CETYL-TRIMETHYL-AMMONIUM | C19 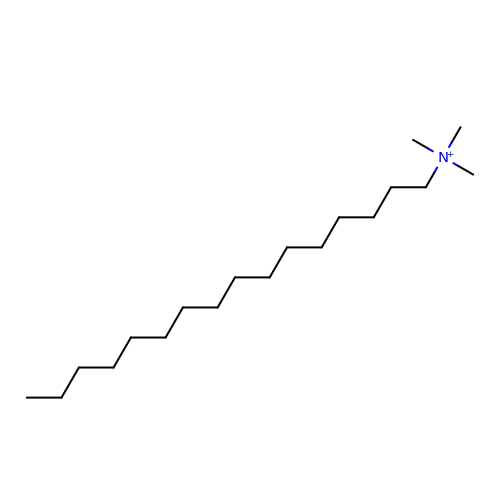H42 N | RLGQACBPNDBWTB-UHFFFAOYSA-N> MNQQGFVISNE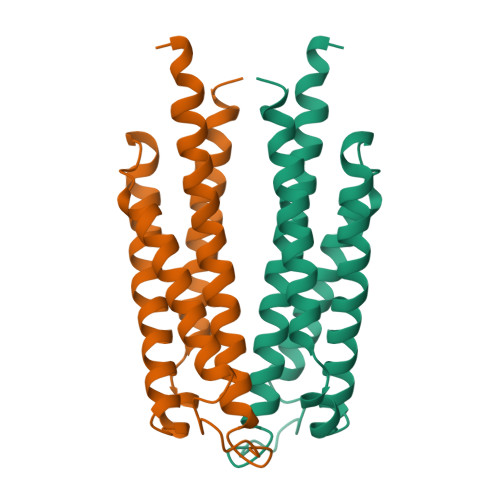LRQQQSELTSTWDLMLQTRINLSRSAARMMMDASNQQSSAKTDLLQNAKTTLAQAAAHYANFKNMTPLPAMAEASANVDEKYQRYQAALAELIQFLDNGNMDAYFAQPTQGMQNALGEALGNYARVSENLYRQTF> DMPVERILEAELAVEPKTETYVEANMGLNPSSPNDPVTNICQAADKQLFTLVEWAKRIPHFSELPLDDQVILLRAGWNELLIASFSHRSIAVKDGILLATGLHVHRNSAHSAGVGAIFDRVLTELVSKMRDMQMDKTELGCLRAIVLFNPDSKGLSNPAEVEALREKVYASLEAYCKHKYPEQPGRF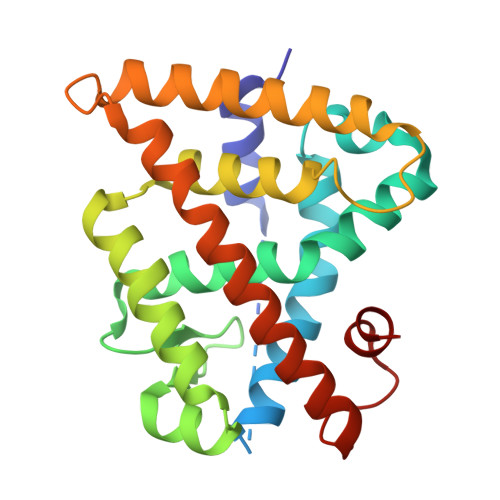AKLLLRLPALRSIGLKCLEHLFFFKLIGDTPIDTFLMEMLE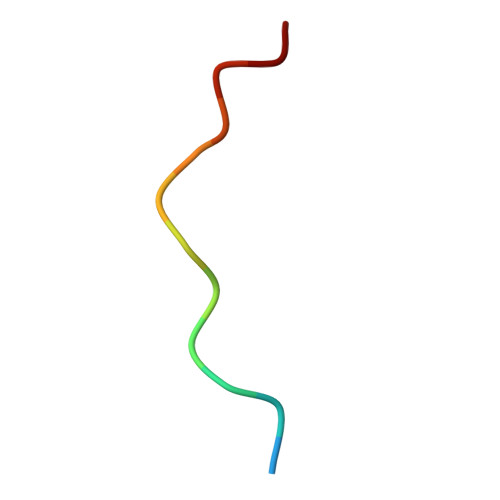> RVPPPPPPPPPLP> MGGKASEAVTIAFRFPHRTTFLVKQNVGQKLNKGHQTFWQLVAGGWLFFLLINR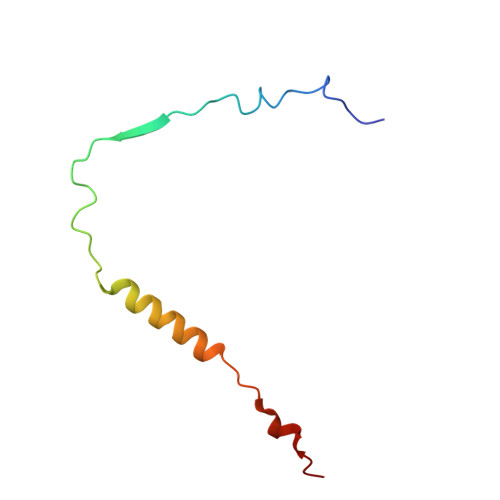TSFKPKLAAPKV> GIGKFLHAA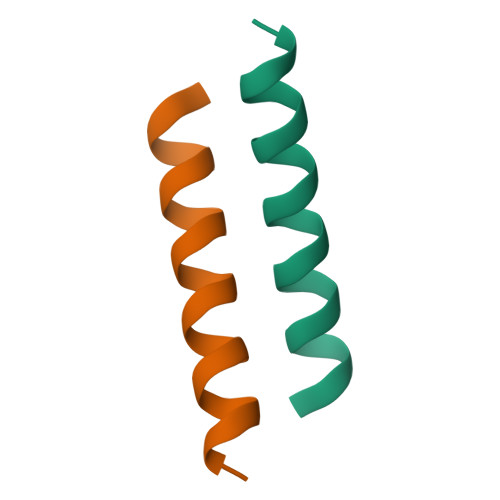KKFAKAFVAEIMNS>MPDVDWNMLRGNATQAAAGAYVPYSRFAVGAAALVDDGRVVTGCNVQNVSYGLTLCAECAVVCALHSTGGGRLLALACVDGHG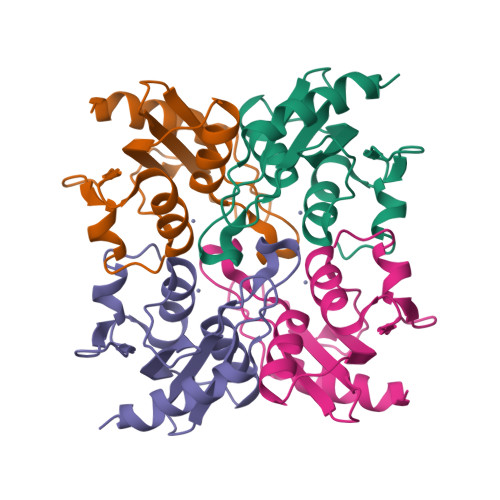SVLMPCGRCRQVLLEHGGSELLIDHPVRPRRLGDLLPDAFGLDDLPRERR[2x]>MGHHHHHHAENLYFQGHMKAVVLRSFGEAGNLKMETMPMPRPGRGEVLLRVHACGVCYHDVINRRGNLPRTSVPAILGHEAAGEVIEVGPDTPGWKTGDRAATLQRMSCGDCALCRSGRNSLCKTDNRFFGEELPGGYAQFMVAPVGGLGRVPASLPWNEAATVCCTTGTAVHTVRTRGKVRAGETVLITGASGGVGLSSVQLARLDGARVIAVTSSEAKVQALKEAGADEVIVSRGLDFASDVRKRTQGAGVDVAVEIVGSATFDQT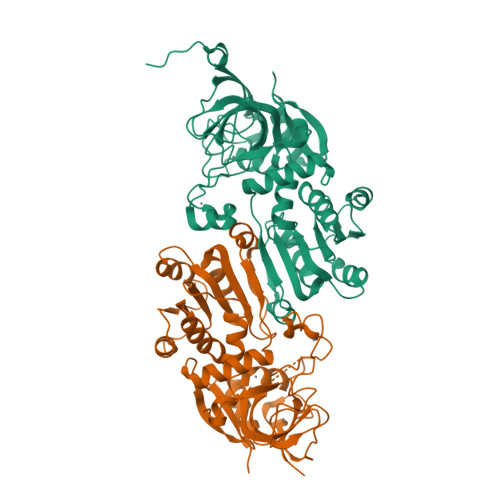LKSMAPGGRVVVVGNLESGMVQLNPGLVIVKELEILGAYATTQAELDEALRLTATGGVRQFVTDAVPLAEAAKAHFRLENREVAGRLVLVPPEA[4x]>[4x]DLSGIISRDQF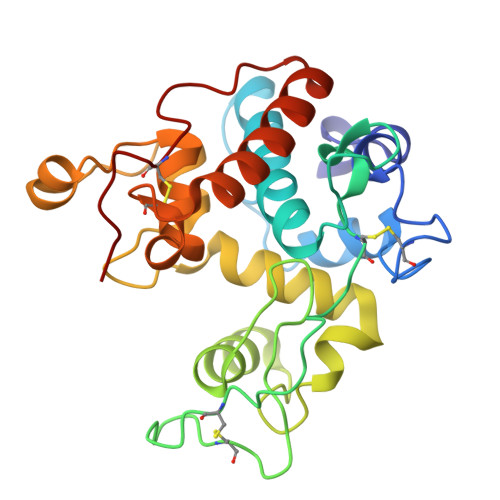YKMLKHMNDNDCHAVGFFTYDAFITAAKSFPSFGNTGDLAMRKKEIAAFFGQTSHETTGGWSGAPDGANTWGYCYKEEIDKSDPHCDSNNLEWPCAPGKFYYGRGPMMLSWNYNYGPCGRDLGLELLKNPDVASSDPVIAFKTAIWFWMTPQAPKPSCHDVITDQWEPSAADISAGRLPGYGVITNIINGGLECAGRDVAKVQDRISFYTRYCGMFGVDPGSNIDCDNQRPFN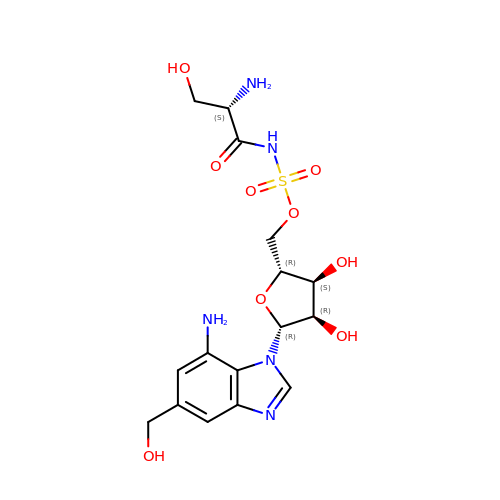[(2~{R},3~{S},4~{R},5~{R})-5-[7-azanyl-5-(hydroxymethyl)benzimidazol-1-yl]-3,4-bis(oxidanyl)oxolan-2-yl]methyl ~{N}-[(2~{S})-2-azanyl-3-oxidanyl-propanoyl]sulfamate | C16 H23 N5 O9 S | YZMBOMBSTSCXHY-LMOQKQACSA-N>GSSCGNDESDPDSTVTIAMATVEKQPQYDAPYLVLDNGEKLWVVQHIVPYRDLKAGERIFGNYSFLEAGESGFAYNIRLNDYTLVPVQKIIGLNPDNMDSIGNMKVQIKDMWPSDDYLNVRFMLNFPSPQKPILNLVVNEMIPWTKDGYAHLELRYNNNGSQGRLVPGMVSFK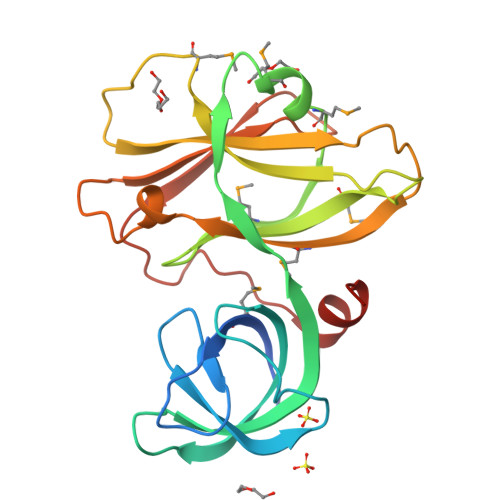LDDYSPENSELKGIKVLVNPVDGEEKTYIFSYPLTGEDVPGFNPLDLAELK[2x]> GPLGSCSSPQVEIPTTYSPEKIAQLQVYVNPIAVARDGMEKRLQGLIADQNWVDTQTYIHGPLGQLRRDMLGLASSLLPKDQDKAKTLAKEVFGH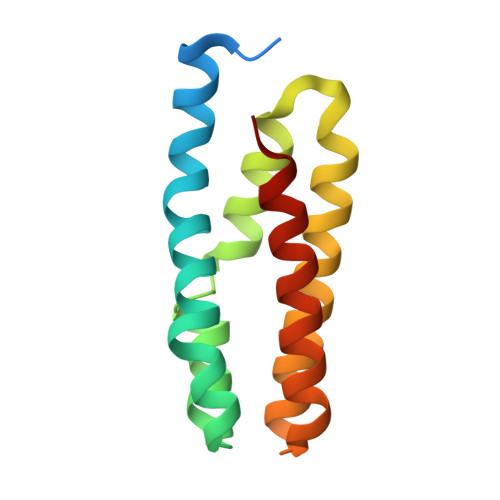LERLDAAAKDRNGSQAKIQYQEALADFDSFLNLLPQAS>MKTIGILGGMGPLATAELFRRIVIKTPAKRDQEHPKVIIFNNPQIPDRTAYILGKGEDPRPQLIWTAKRLEECGADFIIMPCNTAHAFVEDIRKAIKIPIISMIEETAKKVKELGFKKAGLLATTGTIVSGVYEKEFSKYGVEIMTPTEDEQKDVMRGIYEGVKAGNLKLG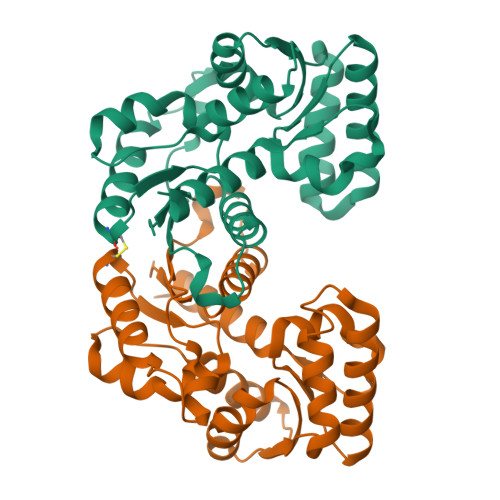RELLLKTAKILEERGAECIIAGCTEVSVVLKQDDLKVPLIDPMDVIAEVAVKVALEK[2x]>DEALSRHFNELRTMGETLKYSEDLDFILSDNSMTTPEHRRNNMLRLCLDMMNNEDLCQYIVKYRHREVWEWCFQGTDPKQKVTSLLQCFIADKIPLLRHDKRWAMLSLENFILPLATDEVFPKKIAGSRLVKLNYQDLLRKLKFTNTCEYALYIWATYLLYTEAVYGAVPALARLISRGQLKDWDTACSLLENNIVAAPSGSDIEEYAQAFQTLAGLSREKLTNEGVLKCLIKLTNHTTVLELSADLL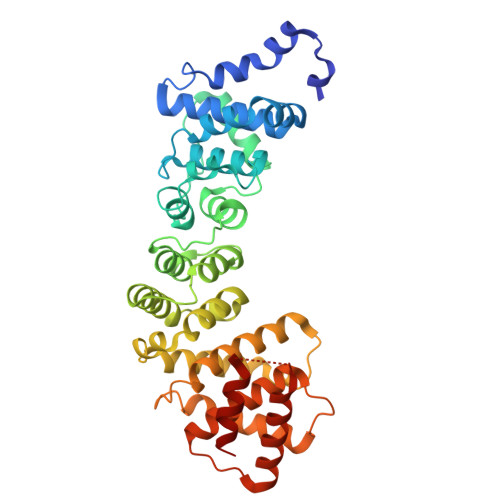PSLVRSLAMSVQLHQNNIVSSISEIKTNLLILQLGLLLNIVSEATTAASTEELTNFGAVFRSVFVKKPTEMSFVLQLFLLVYAYSAGAAGVQLPPAEADFLKSELEAFATDVSSYNHNIHTRITRVLETL[2x]>CCGGCGC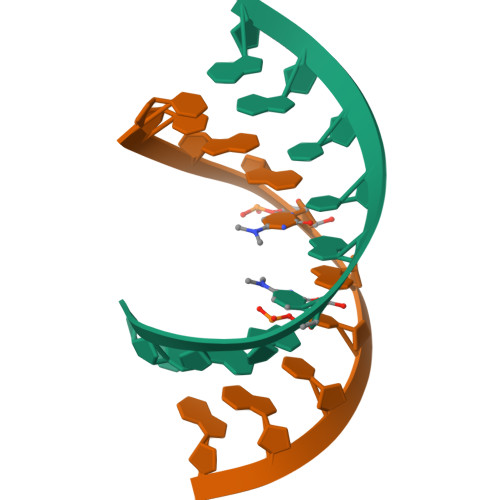CGG[2x]> GSHMTAYTAERQPERDITPVNDETMQEINT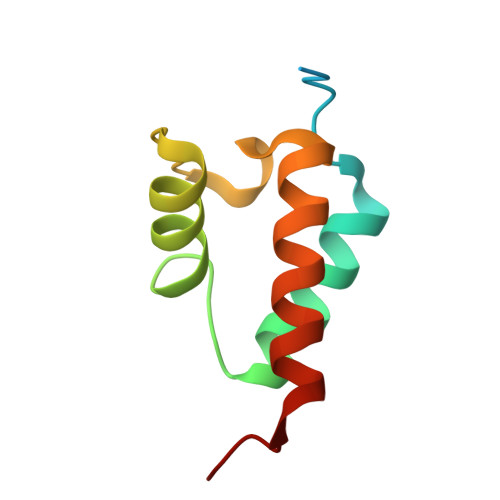LLIALDKTWDDDLLPLCSQIFRRDIRASSELTQAEAVKALGFLKQKAAEQKVAA The final step of PG biosynthesis in Mtb is catalyzed by two different classes of enzymes, namely the D,D-transpeptidases (also known as Penicillin Binding Proteins – PBPs) and L,D-transpeptidases (Ldts). Conversely, Ldts catalyze the crosslinking of disaccharyl-tetrapeptide polymers by forming a transpeptide bond between the third amino acid in adjacent stem peptides thereby generating 3 → 3 crosslinkages between mDAP residues. Approximately two-thirds of the linkages in Mtb PG are of 3 → 3 type and their synthesis is catalyzed by the Ldts, highlighting the importance of these non-classical transpeptidases to this pathogen. Mtb lacking LdtMt2 is severely attenuated for growth, virulence, has deformed cell walls and exhibits an increased susceptibility to β-lactams.

In summary, biapenem and tebipenem bind to the outer cavity of LdtMt2 and inactivate the enzyme, ultimately forming the same adduct following degradation. Additional electron density connected to the catalytic Cys354 thiol group and extending to the outer cavity was observed in LdtMt2–biapenem and LdtMt2–tebipenem complexes. The carboxyl substituent at C5 docks in a pocket and accepts hydrogen bonds from the NH groups of His352, Gly353, and Cys354. After a short incubation, the difference between primary peaks of the mass spectra of unreacted LdtMt2 and the biapenem-LdtMt2 complex was Δm/z = 225 Da, which is less than the expected increase for an intact biapenem adduct (Δm/z = 352 Da). After 40 min and up to 24 h, the primary signal differences stabilized at 180 Da (45 Da less than the difference observed after a short incubation). After a 45 min incubation of biapenem and LdtMt2, the difference between mass spectra primary signals stabilized at around a 180 Da, which is 45 Da less than difference observed after a short incubation and closely matches the difference expected (183 Da, step 7). Decarboxylation of the MTOA adduct results in a Δm/z of 140.1 Da, that closely matches the 139.5 Da observed for LdtMt2-biapenem by mass spectrometry. Few biapenem degradation paths exist yielding this observed adduct mass. Thus, this finding provides strong additional evidence supporting the identification of MTOA as the adduct observed in the LdtMt2-biapenem crystal.

>DLLVPKLTASVTDGAVGVTVDAPVSVTAADGVLAAVTMVNDNGRPVAGRLSPDGLRWSTTEQLGYNRRYTLNATALGLGGAATRQLTFQTSSPAHLTMPYVMPGDGEVVGVGEPVAIRFDENIADRGAAEKAIKITTNPPVEGAFYWLNNREVRWRPEHFWKPGTAVDVAVNTYGVDLGEGMFGEDNVQTHFTIGDEVIATADDNTKILTVRVNGEVVKSMPTSMGKDSTPTANGIYIVGSRYKHIIMDSSTYGVPVNSPNGYRTDVDWATQISYSGVFVHSAPWSVGAQGHTNTSHGCLNVSPSNAQWFYDHVKRGDIVEVVNTVGGTLPGIDGLGDWNIPWDQWRAGNAKA[2x]[(5S)-5-amino-5-carboxy-6,6-difluorohexyl](trihydroxy)borate(1-) 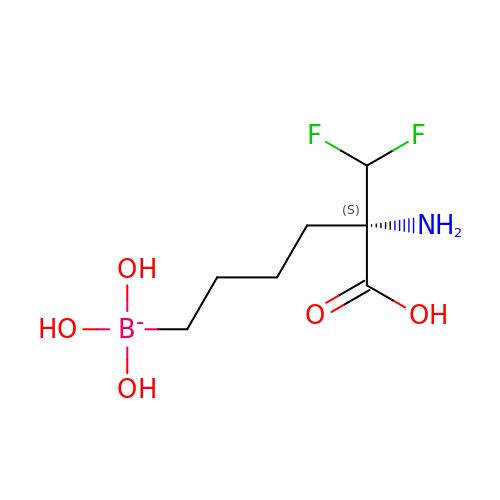| C7 H15 B F2 N O5 | MBESMFYYLXWNTB-SSDOTTSWSA-N The hypothetical protein NP_247299.1 is the gene product of locus MJ0327 in the genomic sequence of the Methanococcus jannaschii genome. Its function is unknown, but on the basis of sequence similarity the NP_247299.1 protein has been assigned to the dinitrogenase iron–molybdenum cofactor family (PF02579). The fold topology of NP_247299.1 resembles a ribonuclease H-like motif, with a three-layer α/β/α architecture.

The crystal structure was determined to 1.7 Å resolution at 100 K using a crystal obtained at 277 K from 100 mM Tris–HCl solution pH 7.0 containing 50%(w/v) PEG 200. The NMR structure of the protein NP_247299.1 in solution at 313 K has been determined and is compared with the X-ray crystal structure, which was also solved in the Joint Center for Structural Genomics (JCSG) at 100 K and at 1.7 Å resolution. The key message is that the two structures of NP_247299.1 determined with current JCSG methodology either in solution at 313 K for NMR data collection or in a single crystal at 100 K show very close coincidence both globally and in residue-by-residue com­parisons. Relatively high displacements are observed for residues 10–15, 30–34, 44–48 and 66–75 in the crystal structure and for residues 35–39, 42–46, 52–56 and 73–75 in the NMR structure. Along the polypeptide chain, high B-value-derived displacements are noted for four segments (residues 10–15, 30–34, 44–48 and 66–74). In particular, for residues 10–15, the electron density is unambiguous and does not show any evidence of the Asp11–Val12 peptide flip indicated by the NMR data. Residues 30–34 did show some minor differences between the initial REFMAC5 model and the rebuilt phenix.refine model, but again there was no indication that the backbone adopts multiple conformations. For residues 36–39, where the NMR data are interpreted as a ‘sliding β-bulge’, the maps are once again unambiguous, without any indication of multiple conformations of the backbone. While there is clear-cut NMR evidence for the presence of two local conformations formed by these six residues, we found no evidence for multiple conformations; the conformer with cis-Pro104 did not refine well and was pushed out of the density in each case. Moreover, the carboxy-terminus hydrogen bonds to Lys36 in the symmetry-related molecule and to two waters, which together appear to stabilize the trans conformation.

> GMINMKVAISMDVDKISNSFEDCKYFLIVRIDDNEVKSTKVIFNDESGKKSIVKENVNAIICKNISEENYKKFSKKIEIYHAEGDDVDKNISLFIEGELSKISNP4-[[(2~{S},3~{R})-1-[(~{E})-3-[5-chloranyl-2-(1,2,3,4-tetrazol-1-yl)phenyl]prop-2-enoyl]-3-phenyl-pyrrolidin-2-yl]carbonylamino]benzoic 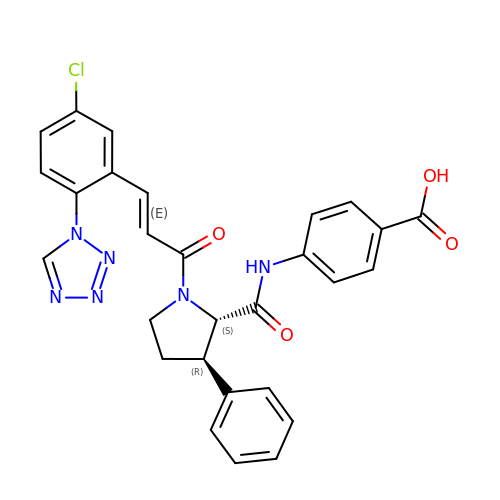acid | C28 H23 Cl N6 O4 | AYEZZMZYYOYMAM-BNNLJGLZSA-N2-[3-[[4,6-bis(chloranyl)-1~{H}-indol-2-yl]methylamino]propylamino]-3~{H}-quinazolin-4-one | C20 H19 Cl2 N5 O | 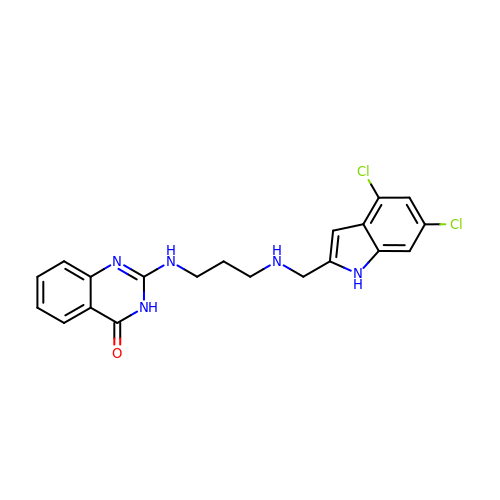NMEFYZKHRBDWLZ-UHFFFAOYSA-N>TERDQMQDHDMTLLMPKSQGRIVVMAVLNRYDSHSANAIIETLASDVFNPEVHYIMIPVGPGHWRGVYLSKPQGGTSDTAYDLELFDPYGPEGAAVLDDYVLDLLNQCGVPKELVNI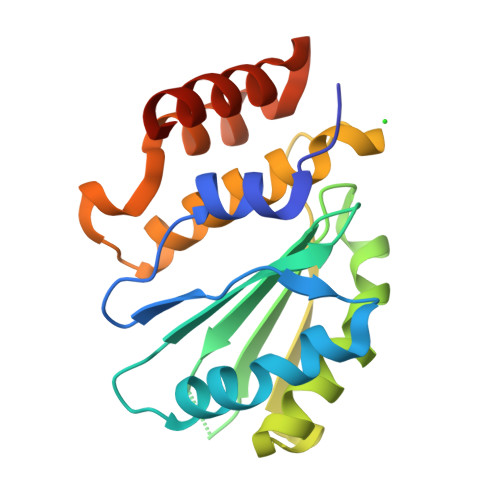RHTGPKHPQGDAYSCGDFTCAYSHKKMKEFGAPEGSYNPILIDTLDNLGNEDNVLRMTTREETRALVDKDRGR[2x]>MGPAFEFAVAMMKRNSSTVKTEYGEFTMLGIYDRWAVLPRHAKPGPTILMNDQEVGVLDAKELVDKDGTNLELTLLKLNRNEKFRDIRGFLAKEEVEVNEAVLAINTSKFPNMYIPVGQVTEYGFLNLGGTPTKRMLMYNFPTRAGQAGGVLMSTGKVLGIHVGGNGHQGFSAALLKHYFNDEQ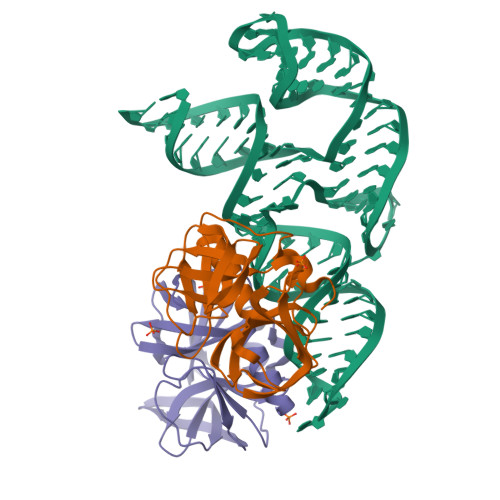LEHHHHHH[2x]>[2x]SNAMRLLVTTLSLIPSIILAAPQLDDSFKNLENKYDGKIGIYTLNTDDKTNIKYNESYHFPICSVFKFLLVGAILDYDMHNQGFLDKKIPINQDDIGKLGYAPITAKNVGKTLTISQLNYAAILSDSPASNILVREL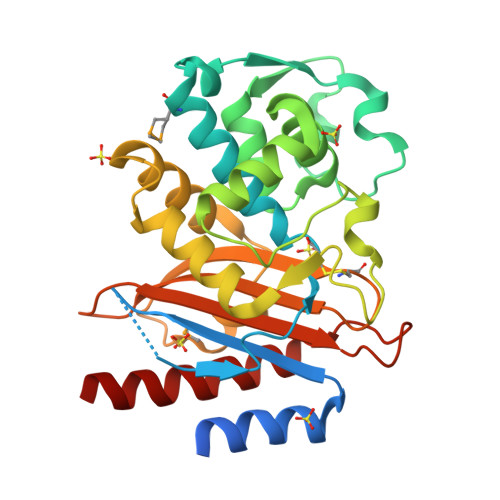GGLQNLNKFIKKLGDNDTIITADEPEINYTQPHSNINKTTPKAITKDIYKLAFGNILDKKHKDIFIKYLQDNNTGANRIAFSMPKDWIIGDKTGTCGQYAATNDVAIIWPKNQQPIALGILYTNPNDKNAPSNEEIIQQAAKLIANDLTNTYK> MAKAHVATLEGNYSDIVLGRVVAFGDTGWNFKEVDMTFIADDADADSKTTLFAGVLVGEDGTPATAAAGVFGVLVDRKVLPGVDHYIGVFEPGEKVPMVLAVRGLTLNQLKLKYADGTAIDAAGIQALEAQGNQVTDKIVGTQF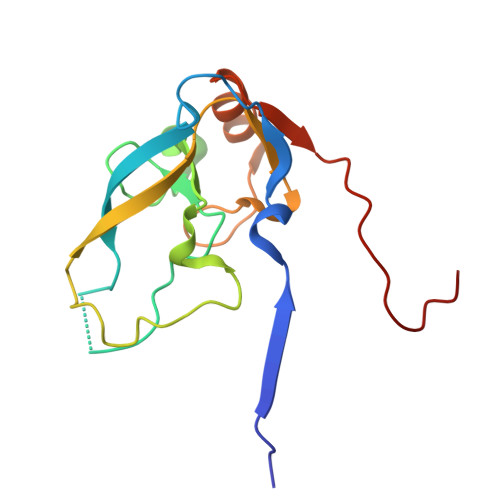IGSVL>EEAELAYLLGELAYKLGEYRIAIRAYRIALKRDPNNAEAWYNLGNAYYKQGDYDEAIEYYQKALELDPNNAEAWYNLGNAYYKQGDYDEAIEYYQKALELDPNNAEAKQNLGNAKQKQG[6x]

We sought to develop a general computational method for de novo designing protein nanoparticles with geometries tailored to present antigens of interest, focusing specifically on the prefusion conformations of the trimeric viral glycoproteins HIV-1 Env (BG505 SOSIP), influenza hemagglutinin (H1 HA), and respiratory syncytial virus (RSV) F (DS-Cav1). In the first step, we de novo designed antigen-tailored trimers, featuring N termini geometrically matched to the C termini of the viral glycoproteins. In the second step, we generated tetrahedral, octahedral, and icosahedral two-component nanoparticles by designing secondary interfaces between a designed trimer (fusion component) and a de novo homo-oligomer (assembly component). This design approach yielded nanoparticles tailored to present 4, 8, or 20 copies of the viral glycoproteins in defined geometries.

We chose to design our antigen-tailored trimers from monomeric repeat proteins composed of rigidly packed 20- to 50-residue tandem repeat units, as their high stability and tunable length (through variation of repeat number) are desirable properties for the design of protein-based nanomaterials. Geometrically compatible docks (non-clashing termini separation distances of 15 Å or less) were subjected to full Rosetta C3-symmetric interface design and filtering, and twenty-three designs were selected for experimental characterization. Four of the designs that were trimeric and expressed in high yield, 1na0C3_2, 3ltjC3_1v2, 3ltjC3_11, and HR04C3_5v2, were selected for solution small angle X-ray scattering (SAXS) experiments. The proteins exhibited scattering profiles very similar to those computed from the corresponding design models, suggesting similar supramolecular configuration (Figure 2 top panel, third row; metrics in Table 1 and Figure 2—source data 1). Crystals were obtained for the two designs 1na0C3_2 and 3ltjC3_1v2. Structures were determined at resolutions of 2.6 and 2.3 Å, revealing a backbone root mean square deviation (r.m.s.d.) between the design model and structure of 1.4 and 0.8 Å, respectively (Figure 2—figure supplement 3, and Figure 2—figure supplement 3—source data 1, crystallization conditions, structure metrics, and structure-to-model comparisons are described in Materials and Methods). The structures confirmed in both cases that the designed proteins adopt the intended trimeric configurations, and that most of the atomic details at the de novo designed interfaces are recapitulated.>[2x]MTTLTRADWEQRAQNLKIEGRAFIQGEYTAAASGETFDCISPVDGRLLAKVASCDAADAQRAVESARSAFDSGAWSRLAPAKRKATMIRFAGLLEQNAEELALLETLDMGKPISDSLGVDIPGGARALSWSGEAIDKLYDEVAATPHDQLGLVTREPVGVVAAIVPWNFPLMMACWKLGPALSTGNSVVLKPSEKSPLTAIRIAQLAIEAGIPAGVLNVLPGYGHTVGKALALHMDVDTVVFTGSTKIAKQLMIYAGESNMKRVWLEAGGKSPNIVFADAPDLQAAADSAASAIAFNQGEVCTAGSRLLVERSIKDRFLPMVIEALGTWKPGNPLDPATNVGALVDTQQMNTVLSYIAAGHTDGARLVAGGKQILQETGGTYVEPTIFDGVNNAMRIAQEEIFGPVLSVLTFDTAEEAIQIANDTPYGLAAAVWTANLSKAHLTARALRAGSVWVNQYDGGDMTAPFGGFKQSGNGRDKSLHAFDKYTELKSTWIKL

Here, we demonstrate that DC3000 produces IAA and identify an indole-3-acetaldehyde dehydrogenase, AldA, that catalyzes the NAD-dependent formation of IAA from indole-3-acetaldehyde (IAAld). The AldA monomer adopts a canonical aldehyde dehydrogenase fold, which contains an NAD+-binding domain with a Rossmann-fold motif of a central β-sheet (β10-β9-β8-β11-β12) surrounded by α-helices, a mixed α/β domain with the catalytic cysteine residue (Cys302), and an oligomerization domain with a protruding β-sheet (β6-β7-β23). In each structure, two AldA monomers were in the asymmetric unit and packed to form a dimer, which then form a tetramer by crystallographic symmetry. Overall, the biochemical and structural data presented here indicate that in P. syringae strain DC3000 AldA functions as an IAAld dehydrogenase in IAA biosynthesis.

The AldA•NAD+ and AldA•NAD+•IAA crystal structures define the position of the active site between the catalytic and cofactor binding domains. Unambiguous electron density in the AldA•NAD+ and AldA•NAD+•IAA crystal structures identifies the respective ligand binding sites. In the NAD+ binding site, the cofactor is bound in a hydrophobic tunnel. The adenine ring of NAD+ lies in an apolar region that provides multiple van der Waals contacts. The adenine ring also forms two hydrogen bonds between the hydroxyl group of Tyr255 and a water. The adenine-ribose rings provide extensive polar interactions with AldA. The 2’-hydroxyl hydrogen bonds with Lys191 and Glu194. Interactions with Ser193, Ser245, and Trp167 position the phosphate backbone in the binding site. The nicotinamide-ribose forms a bidentate interaction with Glu401 and the nicotinamide ring is bound by a water-mediated interaction with Thr243 and through a hydrogen bond from Glu267. Sequence comparisons show a conserved NAD+ binding site in AldA, AldB and AldC. These interactions place the nicotinamide ring in proximity to the invariant catalytic cysteine (Cys302 in AldA).MnSOD-2 and MnSOD-3 are homologous proteins and are both synthesized as precursors with N-terminal mitochondrial targeting signals. Here we present the structures of the two MnSODs which are strikingly similar to that from human. Gel-filtration chromatography indicated that the pure proteins were tetrameric, a result that was confirmed by analytical ultracentrifugation (results not shown). Similar to other reported MnSODs, the tetrameric quaternary structure in MnSOD-2 and MnSOD-3 is accomplished through interactions of the N-domain α-hairpin.

Extensive studies have revealed differential expression patterns, with MnSOD-2 emerging as the major constitutive MnSOD. Specific activity was estimated for MnSOD-2 as 3622 ± 80 U mg−1 per manganese and for MnSOD-3 as 3261 ± 26 U mg−1 per manganese; the proteins were 60 and 100% metallated with mangan­ese, respectively. The C. elegans MnSODs are structurally similar to the human enzyme; superposition of all the Cα atoms of MnSOD-2 and MnSOD-3 with human SOD gives root-mean-square-deviations of 0.5 and 0.8 Å, respectively. One chain (chain C) in each SOD asymmetric unit was found to contain electron density corresponding to the N-terminal methionine residue. Two cis-prolines (Pro16) are present in each chain in common with other MnSODs. Two residues, Asn141 and Lys169 (MnSOD-2 numbering), have torsion angles in less favourable regions of the Ramachandran diagram. Asn141 adopts ϕ and ψ angles of 52° and −125°, respectively, such that its carbonyl group lies parallel to the indole ring of Trp160 with the oxygen forming a hydrogen bond to N∊. Lys169 adopts ϕ and ψ angles of 54° and −133°, with its carbonyl group packing parallel to the Tyr165 side-chain ring. Substrate access to the metal is controlled by residues from both subunits (not shown), while two residues from the other subunit forming the dimer contribute to the stability of the active site. One of these residues, Glu161 (MnSOD-2 numbering), is highly conserved and may contribute to intersubunit communication during catalysis.

>[2x]MKHSLPDLPYDYADLEPVISHEIMQLHHQKHHATYVNNLNQIEEKLHEAVSKGNVKEAIALQPALKFNGGGHINHSIFWTNLAKDGGEPSAELLTAIKSDFGSLDNLQKQLSASTVAVQGSGWGWLGYCPKGKILKVATCANQDPLEATTGLVPLFGIDVWEHAYYLQYKNVRPDYVNAIWKIANWKNVSERFAKAQQ(2E)-3-{5-[(2,4-diaminopyrimidin-5-yl)methyl]-2,3-dimethoxyphenyl}-1-[(1R)-1-(2-methylprop-1-en-1-yl)phthalazin-2(1H)-yl]prop-2-en-1-one | C28 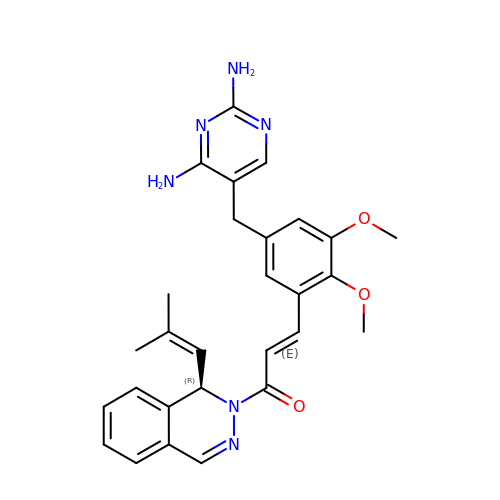H30 N6 O3 | LEKSMFBSZBQJBZ-JJNABOQBSA-N> MRGSHHHHHHTDPQGDAAQKTDTSHHDQDHPTFNKITPNLAEFAFSLYRQLAHQSNSTNIFFSPVSIATAFAMLSLGTKADTHDEILEGLNFNLTEIPEAQIHEGFQELLRTLNQPDSQLQLTTGNGLFLSEGLKLVDKFLEDVKKLYHSEAFTVNFGDTEEAKKQINDYVEKGTQGKIVDLVKELDRDTVFALVNYIFFKGKWERPFEVKDTEEEDFHVDQVTTVKVPMMKRLGMFNIQHSKKLSSWVLLMKYLGNATAIFFLPDEGKLQHLENELTHDIITKFLENEDRRSASLHLPKLSITGTYDLKSVLGQLGITKVFSNGADLSGVTEEAPLKLSKAVHKAVLTIDEKGTEAAGAMFLEAIPMSIPPEVKFNKPFVFLMIEQNTKSPLFMGKVVNPTQK

Ninety‐five per cent of severe deficiency results from the “Z” allele (Glu342Lys) that perturbs the folding of α1‐antitrypsin resulting in the secretion of only 15% of the mature protein. The Z mutation lies at the head of strand 5 of β‐sheet A of α1‐antitrypsin. It perturbs the local environment, allowing population of an unstable intermediate that we have termed M* in which β‐sheet A opens and the upper part of helix F unwinds. Polymerisation from this state involves insertion of the RCL into β‐sheet A with a domain‐swap of the C‐terminal region providing the inter‐subunit linkage.

A high‐resolution crystal structure of α1‐antitrypsin complexed with the lead compound GSK716 was generated by soaking compound into apo α1‐antitrypsin crystals. The structure reveals that interaction with the compound induces the formation of a cryptic binding site that is not evident in apo structures, at the top of β‐sheet A behind strand 5. This region is referred to as the “breach” as it is the point at which the reactive centre loop first inserts during protease inhibition, and includes the site of the Z (Glu342Lys) mutation. The structure reveals that the 2‐oxindole ring of GSK716 stacks with the side chain of Trp194 whilst the carbonyl group forms a hydrogen bond with the mainchain Trp194. Trp194 adopts a new position due to rearrangement of residues Gly192 to Thr203 consistent with the change in intrinsic tryptophan fluorescence induced by binding. The phenyl ring and the propyl chain occupy two highly hydrophobic pockets. Hydrogen bonds are formed between the GSK716 hydroxyl group and the Leu291 backbone, the amide nitrogen hydrogen and the backbone carbonyl oxygen of Pro289, and between the amide carbonyl and the Tyr 244 hydroxyl group. This causes displacement of residues Thr339 to Ser 359 of strand 5A relative to the apoprotein. The co‐crystal structure with α1‐antitrypsin demonstrates that the small molecule ameliorates the effect of the Glu342Lys (Z) mutation by: (i) optimisation of hydrophobic packing in the breach region; (ii) formation of hydrogen bonds with buried polar atoms; and (iii) displacement of the backbone at the top of strand 5A into a configuration less compatible with partial loop insertion. GSK716 stabilises the partially folded α1‐antitrypsin or the fully folded but labile aberrant native form. This mode of action is compatible with the lack of binding of GSK716 to polymers, in which partial or complete insertion of the reactive centre loop completes a β‐hairpin turn and so occludes the compound binding site.>[4x]CGADSQGLVVSFYTPATDGATFTAIAQRCNQQFGGRFTIAQVSLPRSPNEQRLQLARRLTGNDRTLDVMALDVVWTAEFAEAGWALPLSDDPAGLAENDAVADTL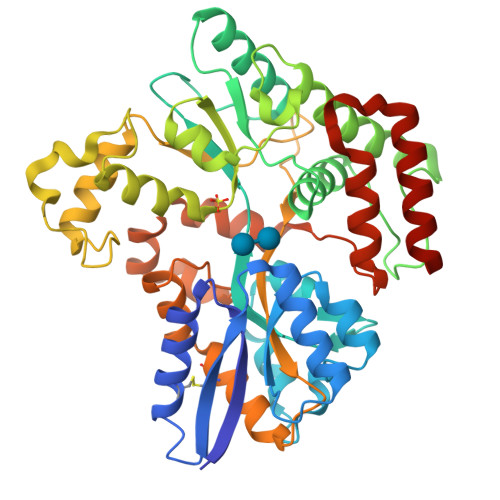PGPLATAGWNHKLYAAPVTTNTQLLWYRPDLVNSPPTDWNAMIAEAARLHAAGEPSWIAVQANQGEGLVVWFNTLLVSAGGSVLSEDGRHVTLTDTPAHRAATVSALQILKSVATTPGADPSITRTEEGSARLAFEQGKAALEVNWPFVFASMLENAVKGGVPFLPLNRIPQLAGSINDIGTFTPSDEQFRIAYDASQQVFGFAPYPAVAPGQPAKVTIGGLNLAVAKTTRHRAEAFEAVRCLRDQHNQRYVSLEGGLPAVRASLYSDPQFQAKYPMHAIIRQQLTDAAVRPATPVYQALSIRLAAVLSPITEIDPESTADELAAQAQKAIDGMGLLP Cryptophyte algae have a unique phycobiliprotein light-harvesting antenna that fills a spectral gap in chlorophyll absorption from photosystems. We show that the cryptophyte Hemiselmis andersenii expresses an energetically complex antenna comprising three distinct spectrotypes of phycobiliprotein, each composed of two αβ protomers but with different quaternary structures arising from a diverse α subunit family. We report crystal structures of the major phycobiliprotein from each spectrotype. We propose that the macromolecular organization of the cryptophyte antenna consists of bulk open and open-braced forms that transfer excitations to photosystems via this bridging closed form phycobiliprotein.

Four new structures of HaPE555 were determined (resolutions: 1.57 Å, 1.67 Å, 1.73 Å and 1.95 Å). The largest peak of HaPE555 (555 A) is by far the most abundant PBP constituting approximately 63% of the overall protein complement (with other HaPE555 spectrotype peaks contributing 8%). All five crystal forms of protein HaPE555 are constructed from continuous filaments of PBPs, which are organized into two-dimensional rafts. The filaments are generated via knobs-into-holes packing but differ in the distances between adjacent molecules along the filament (having either tight or loose interfaces). This packing brings the chromophores of neighboring PBPs closer together increasing the possibility of energy transfer. The bulk antenna proteins, HaPE555 and HaPE560, are densely packed to form a concentrated glass of proteins as evidenced by electron micrographs and FRAP experiments. It is also possible that the rafts of HaPE555 filaments seen in all crystal forms are part of the organizing principle of the antenna architecture. We have shown that HaPE555 and HaPE560 form the bulk of the light harvesting antenna (roughly 6/7 of the PBPs) and capture the highest energy photons. Thus, HaPE555 and HaPE560 have evolved to capture photons that would be otherwise lost by the integral membrane photosystems: they plug a spectral hole.

>[4x]AMKKDSKAPCVEVFDERDGCKAAGTQKASGDDGFCVKVSMKAIGFNAAEAASVTKNYGIKRFGAKSV;>[4x]MLDAFSKVITSADGKAAYVGGADLQALKKFVSEGNKRMDSVNAIVSNASCIVSDSVSGMVCENPSLIAPNGGVYTNRKMAACLRDAEIILRYVSYSLLSGDSSVLEDRCLNGLKETYASLGVPAAGNARTISIMKATVIGFITNNSQQKKLSTPAGDCSALASEVGGYFDKVSSALA;>AMKKDSKAPCVEVFDERDGCKAAGTQKASGDDGFCVKVSMKAIKMNAAEATSVTKNYNTKLL[4x]>MPNIKIFSGSSHQDLSQKIADRLGLELGKVVTKKFSNQETCVEIGESVRGEDVYIVQSGCGEINDNLMELLIMINACKIASASRVTAVIPCFPYARQDKKDKSRAPISAK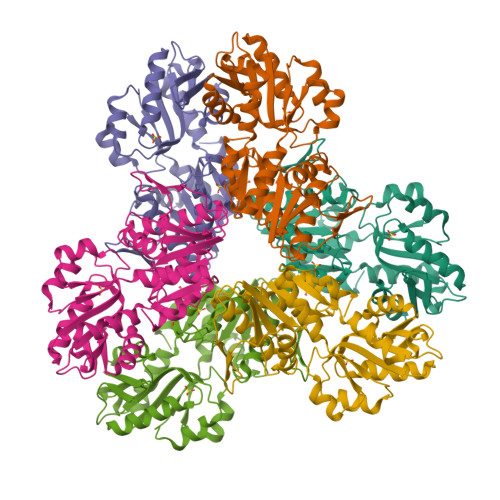LVANMLSVAGADHIITMDLHASQIQGFFDIPVDNLYAEPAVLKWIRENISEWRNCTIVSPDAGGAKRVTSIADRLNVDFALIHKERKKANEVDRMVLVGDVKDRVAILVDDMADTCGTICHAADKLLSAGATRVYAILTHGIFSGPAISRINNACFEAVVVTNTIPQEDKMKHCSKIQVIDISMILAEAIRRTHNGESVSYLFSHVPLLEHHHHHH[2x]> MRGNIRVYCRIRPALKNLENSDTSLINVNEFDDNSGVQSMEVTKIQNTAQVHEFKFDKIFDQQDTNVDVFKEVGQLVQSSLDGYNVCIFAYGQTGSGKTFTMLNPGDGIIPSTISHIFNWINKLKTKGWDYKVNCEFIEIYNENIVDLLRSDNNNKEDTSIGLKHEIRHDQETKTTTITNVT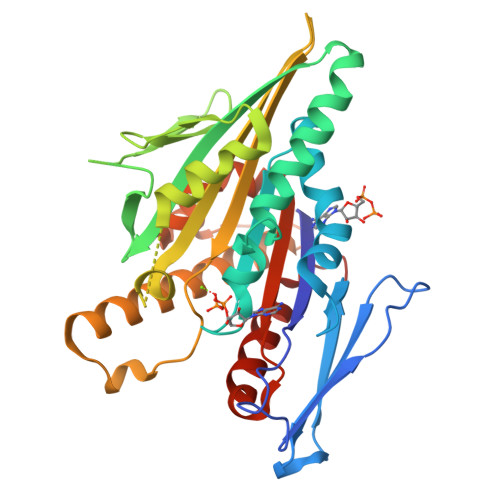SCKLESEEMVEIILKKANKLRSTASTASNEHSSASHSIFIIHLSGSNAKTGAHSYGTLNLVDLAGSERINVSQVVGDRLRETQNINKSLSCLGDVIHALGQPDSTKRHIPFRNSKLTYLLQYSLTGDSKTLMFVNISPSSSHINETLNSLRFASKVNSTRLVSRK> MANSGEEKLKLYSYWRSSCAHRVRIALALKGLDYEYIPVNLLKGDQFDSDFKKINPMGTVPALVDGDVVINDSFAIIMYLDEKYPEPPLLPRDLHKRAVNYQAMSIVLSGIQPHQN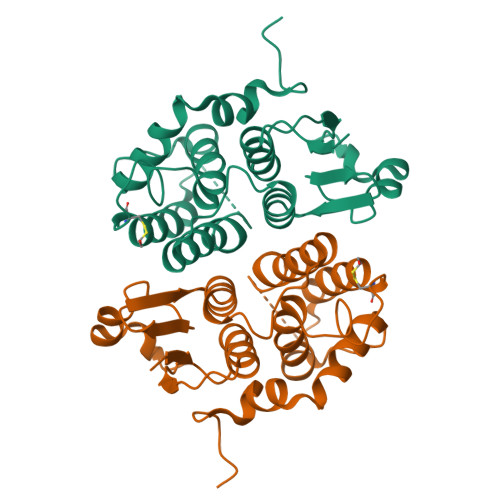LAVIRYIEEKINVEEKTAWVNNAITKGFTALEKLLVNCAGKHATGDEIYLADLFLAPQIHGAINRFQINMEPYPTLAKCYESYNELPAFQNALPEKQPDAPSSTI>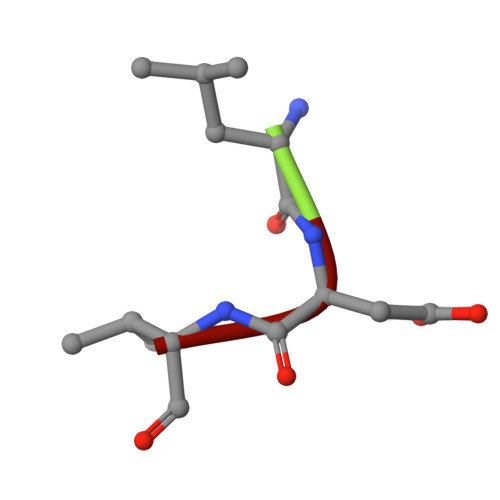 LDV>MSQSPAFGPRRGSSPRGAAGAAARRNESQDYLLMDSELGEDGCPQAPLPCYGYYPCFRGSDNRLAHRRQTVLREKGRRLANRGPAYMFSDRSTSLSIEEERFLDAAEYGNIPVVRKMLEECHSLNVNCVDYMGQNALQLAVANEHLEITELLLKKENLSRVGDALLLAISKGYVRIVEAILSHPAFAEGKRLATSPSQSELQQDDFYAYDEDGTRFSHDVTPIILAAHCQEYEIVHTLLRKGARIERPHDYFCKCNDCNQKQKHDSFSHSRSRINAYKGLASPAYLSLSSEDPVMTALELSNELAVLANIEKEFKNDYKKLSMQCKDFVVGLLDLCRNTEEVEAILNGDVETLQSGDHGRPNLSRLKLAIKYEVKKFVAHPNCQQQLLSIWYENLSGLRQQTMAVKFLVVLAVAIGLPFLALIYWFAPCSKMGKIMRGPFMKFVAHAASFTIFLGLLVMNAADRFEGTKLLPNETSTDNAKQLFRMKTSCFSWMEMLIISWVIGMIWAECKEIWTQGPKEYLFELWNMLDFGMLAIFAASFIARFMAFWHASKAQSIIDANDTLKDLTKVTLGDNVKYYNLARIKWDPSDPQIISEGLYAIAVVLSFSRIAYILPANESFGPLQISLGRTVKDIFKFMVIFIMVFVAFMIGMFNLYSYYIGAKQNEAFTTVEESFKTLFWAIFGLSEVKSVVINYNHKFIENIGYVLYGVYNVTMVIVLLNMLIAMINSSFQEIEDDADVEWKFARAKLWFSYFEEGRTLPVPFNLVPSPKSLFYLLLKLKKWISELFQGHKKGFQEDAEMNKINEEKKLGILGSHEDLSKLSLDKKQVGHNKQPSIRSSEDFHLNSFNNPPRQYQKIMKRLIKRYVLQAQIDK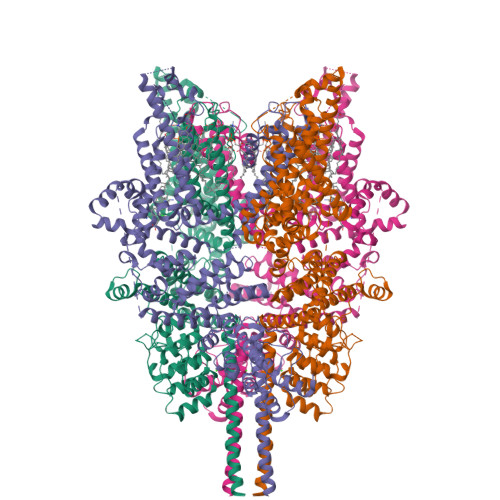ESDEVNEGELKEIKQDISSLRYELLEEKSQNTEDLAELIRELGEKLSMEPNQEETNR[4x]Group A Streptococcus (GAS) is a strict human pathogen possessing a unique pathogenic trait that utilizes the cooperative activity of NAD+-glycohydrolase (NADase) and Streptolysin O (SLO) to enhance its virulence. SLO is a pore-forming toxin belonging to the family of cholesterol-dependent cytolysins (CDCs) and can disrupt eukaryotic cell membranes with its cytolytic activity. SLO is required for the delivery of the effector NADase into the host cytosol in a pore-formation-independent process termed cytolysin-mediated translocation (CMT). The translocated NADase exerts its cytotoxic effects by hydrolyzing β-NAD+ into nicotinamide and ADP-ribose, resulting in cell death through β-NAD+ depletion, and promotion of the intracellular survival of GAS within macrophages, epithelial cells, and endothelial cells.

Analysis of the elution profiles of size exclusion chromatography (SEC) revealed the dynamic N-terminal region of SLO (residues 35-105) is dispensable for binding to the C-terminal enzymatic domain of NADase. Diffraction-quality crystals of C-terminally His-tagged NADase193-451,G330D in complex with tag-free SLO106-574 were produced, and the crystal structure of this complex was determined to a resolution of 2.45 Å by molecular replacement. Within the crystallographic asymmetric unit, two copies of the complex are present, with each complex consisting of NADase193-451,G330D and SLO106-574 at a 1:1 molar ratio, consistent with the reported solution stoichiometry. The overall structure of the NADase193-451,G330D/SLO106-574 heterodimer exhibits an elongated shape with the C-terminal domain 4 of SLO bound to the C-terminal enzymatic domain of NADase. A common polymorphism G330D, with the presence of aspartate instead of glycine at position 330 of NADase, lacks detectable NADase activity. The buried surface area of the complex is ~863 Å2, which is at the smaller end of the range of buried surface area measures of typical protein complexes. Among the interacting residues, NADase residue D315 forms the only salt bridge with SLO residue R531. The elution profile shows NADaseD315R did not co-elute with SLO, indicating the disruption of complex formation. The SEC profile showed NADaseD315R and SLOR531D co-eluted in a single peak at the same elution volume as the wild-type NADase/SLO complex, indicating NADaseD315R/SLOR531D restores the ionic interaction required for complex formation.

>[2x]MGNMERDLFEKKFKEIKDKWVTDKQADEFIETADKYADKAVQMSAVASRAEYYRMYVSRKYHYKKEFVEKLKQVYKESGASHVTSKKDLMLAFDDAKRKSTIGRQENGLFVTSFAEDMALLFTDQGKLKSADQIENIKDVDSGKYSDGVYQYEYDSELTKNIDKLGYIRTASGDTPRANSLNIPGCQTWSGKHIENSESELIFPSISVKDLKSKAVLAEIDAKGYFEIIDPTIIAPNGDHKKVTGRFKIKKMQDRMQDRKLEHHHHHH;>[2x]MASEDHTEEINDKIYSLNYNELEVLAKNGETIENFVPKEGVKKADKFIVIERKKKNINTTPVDISIIDSVTDRTYPAALQLANKGFTENKPDAVVTKRNPQKIHIDLPGMGDKATVEVNDPTYANVSTAIDNLVNQWHDNYSGGNTLPARTQYTESMVYSKSQIEAALNVNSKILDGTLGIDFKSISKGEKKVMIAAYKQIFYTVSANLPNNPADVFDKSVTFKELQRKGVSNEAPPLFVSNVAYGRTVFVKLETSSKSNDVEAAFSAALKGTDVKTNGKYSDILENSSFTAVVLGGDAAEHNKVVTKDFDVIRNVIKDNATFSRKNPAYPISYTSVFLKNNKIAGVNNRSEYVETTSTEYTSGKINLSHQGAYVAQYEILWDEINYDDKGKEVITKRRWDNNWYSKTSPFSTVIPLGANSRNIRIMARECTGLAWEWWRKVIDERDVKLSKEINVNISGSTLSPYGSITYK> KVFERCELARTLKRLGMDGYRGISLANWMCLAKWESGYNTRATNYNAGDRSTDYGIFQI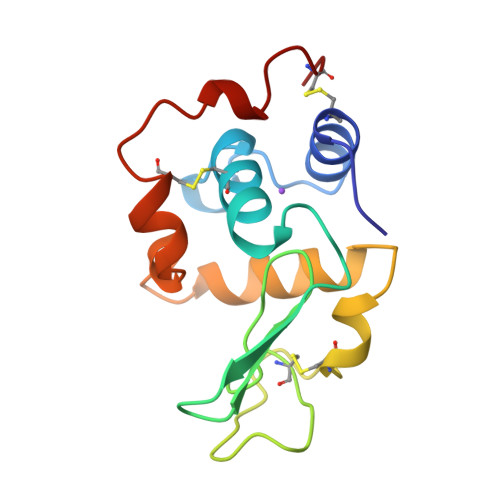NSRYWCNDGKTPGAVNAAHLSCSALLQDNIADAVAAAKRAVRDPQGIRAWVAWRNRCQNRDVRQYVQGCGV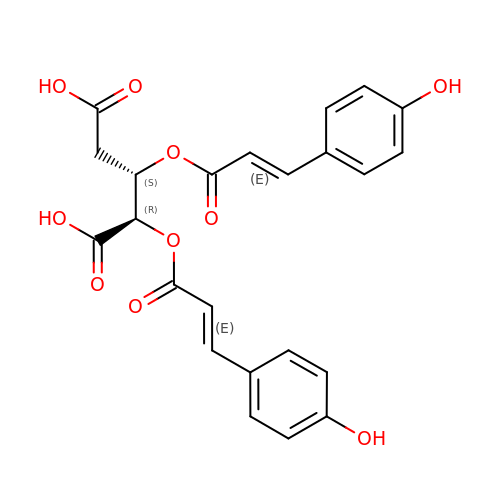2-DEOXY-3,4-BIS-O-[3-(4-HYDROXYPHENYL)PROPANOYL]-L-THREO-PENTARIC ACID | C23 H20 O10 | VJLMRHSHSNLOGC-NOPZTHQXSA-N> MTVLIVTFSRDNESIPLVIKAIEAMGKKAFRFDTDRFPTEVKVDLYSGGQKGGIITDGDQKLELKEVSAVWYRRMRYGLKLPDGMDSQFREASLKECRLSIRGMIASLSGFHLDPIAKVDHANHKQLQLQVARQLGLLIPGTLTSNNPEAVKQFAQEFEATGIVTKMLSQFAIYGDKQEEMVVFTSPVTKEDLDNLEGLQFCPMTFQENIPKALELRITIVGEQIFTAAINSQQLDGAIYDWRKEGRALHQQWQPYDLPKTIEKQLLELMKYFGLNYGAIDMIVTPDERYIFLEINPVGEFFWLELYPPYFPISQAIAEILV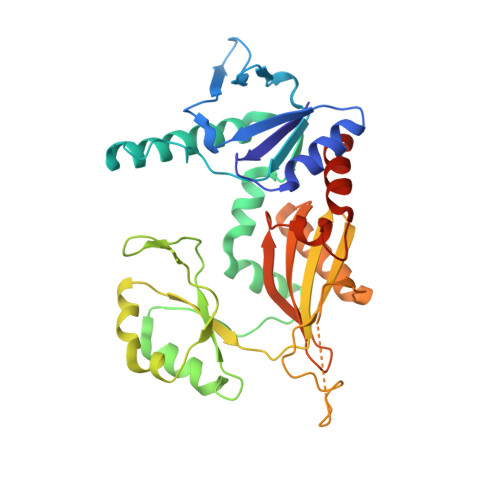NSAAAHHHHHH>MSPLRKTVPEFLAHLKSLPISKIASNDVLTICVGNESADMDSIASAITYSYCQYIYNEGTYSEEKKKGSFIVPIIDIPREDLSLRRDVMYVLEKLKIKEEELFFIEDLKSLKQNVSQGTELNSYLVDNNDTPKNLKNYIDNVVGIIDHHFDLQKHLDAEPRIVKVSGSCSSLVFNYWYEKLQGDREVVMNIAPLLMGAILIDTSNMRRKVEESDKLAIERCQAVLSGAVNEVSAQGLEDSSEFYKEIKSRKNDIKGFSVSDILKKDYKQFNFQGKGHKGLEIGLSSIVKRMSWLFNEHGGEADFVNQCRRF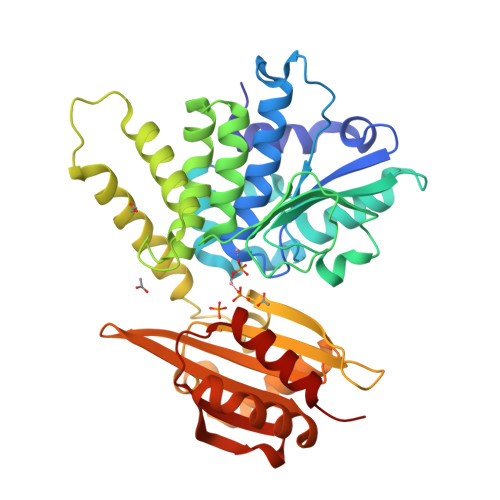QAERGLDVLVLLTSWRKAGDSHRELVILGDSNVVRELIERVSDKLQLQLFGGNLDGGVAMFKQLNVEATRKQVVPYLEEAYSNLEE[2x]The ChAdOx1 viral vector, adapted from chimpanzee adenovirus Y25 (ChAd-Y25), is the basis for the ChAdOx1 nCoV-19 vaccine (AZD1222/Vaxzevria). We have determined the structure of the ChAdOx1 viral vector and used it in state-of-the-art computational simulations to demonstrate an electrostatic interaction mechanism with PF4, which was confirmed experimentally by surface plasmon resonance. Here, we characterized the capsid structure of ChAdOx1 and the primary receptor binding fiber knob protein. We have characterized its primary cell attachment protein, the fiber knob, and show that ChAdOx1, a simian adenovirus, shares considerable structural homology with human adenoviruses.

Adenovirus fiber knob is responsible for the primary virus-cell interaction during infection. To investigate primary ChAdOx1 receptors, we solved the structure of the ChAdOx1 fiber knob receptor. Diffraction data were scaled and merged at 1.59-Å resolution. Superpositioning of the previously reported structure of HAdV-C5 fiber knob and our structure of the ChAdOx1 fiber knob protein show that fold homology is high, despite only 64.86% amino acid sequence homology, including in the loops, with a root mean square deviation of 1.4 Å. There is much lower homology between ChAdOx1 and HAdV-B35 fiber knob. The core fold is similar, but the loops are divergent. ChAdOx1 and HAdV-C5 were both predicted to form numerous polar contacts with CAR, with HAdV-B35 forming very few. HAdV-C5 remains the strongest known CAR-binding adenovirus with an equilibrium binding constant (KD) of 0.06 nM, with ChAdOx1 binding at 7.16 nM, not as strong as HAdV-C5 due to a slower on rate (Ka). To validate these predicted CAR interactions, we performed SPR of ChAdOx1, HAdV-C5, and HAdV-B35 fiber knob proteins binding CAR or CD46. This confirmed that HAdV-C5 and ChAdOx1 fiber knobs bind strongly to CAR but not CD46. A similar analysis in CHO-BC1 cells, expressing CD46-BC1 isoform but no other known primary adenovirus receptors, determined that HAdV-B35, had a strong CD46 interaction, while HAdV-C5and ChAdOx1 fiber knobs did not have a measurable ability to prevent anti-CD46 antibody binding. These experiments, summarized in Fig. 3D, are robust evidence that ChAdOx1 uses CAR as a primary receptor, not CD46 or DSG2.

>[12x]KLTLWTTPDPSPNCQLLSDRDAKFTLCLTKCGSQILGTVAVAAVTVGSALNPINDTVKSAIVFLRFDSDGVLMSNSSMVGDYWNFREGQTTQSVAYTNAVGFMPNLGAYPKTQSKTPKNSIVSQVYLNGETTMPMTLTITFNGTDEKDTTPVSTYSMTFTWQWTGDYKDKNITFATNSFTFSYMAQE> AVSRLLLPSRVRHSYTGKMGAVFIFVGALTVLFGAIA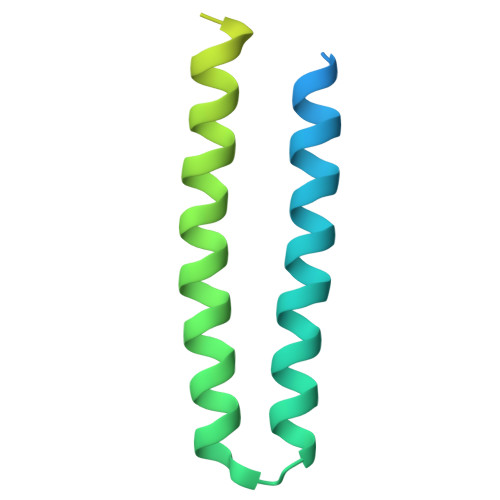YGEVTAAAATGDAAAVQEAAVSAILGLIILLGINLGLVAATLFGDTAASLSTLAAKASRMGDGDLDVELETRREDEIGDLYAAFDEMRQSVRTSLEDHHHHHHH> GEGKEDAFSKLKE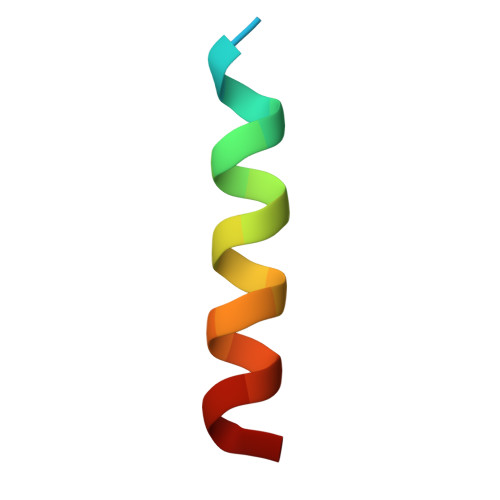KFMNELHK> EYSGPKLEDGKVTISFMKELMQWYKDQKKLHRKCAYQILVQVKEVLSKLSTLVETTLKETEKITVCGDTHGQFYDLLNIFELNGLPSETNPYIFNGDFVDRGSFSVEVILTLFGFKLLYPDHFHLLRGNHETDNMNQIYGFEGEVKAKYTAQMYELFSEVFEWLPLAQCINGKVLIMHGGLFSEDGVTLDDIRKIERNRQPPDSGPMCDLLWSDPQPQNGRSISKRGVSCQFGPDVTKAFLEENNLDYI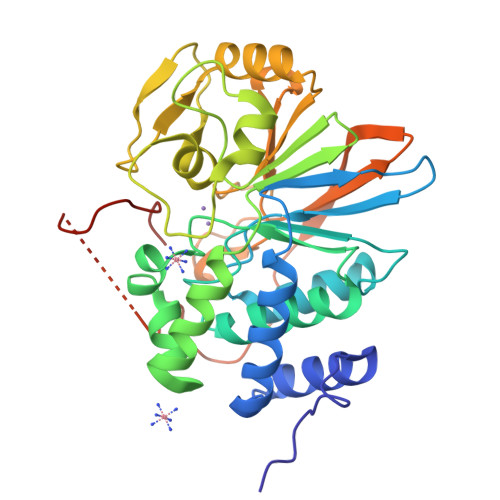IRSHEVKAEGYEVAHGGRCVTVFSAPNYCDQMGNKASYIHLQGSDLRPQFHQFTAVPHPNVKPMAYANTLLQLGMMGSGSGSASRSVWDHIEVEDDEDETH>[30x]MSMYTTAQLLAANEQKFKFDPLFLRLFFRESYPFTTEKVYLSQIPGLVNMALYVSPIVSGEVIRSRGGSTSEFTPGYVKPKHEVNPQMTLRRLPDEDPQNLADPAYRRRRIIMQNMRDEELAIAQVEEMQAVSAVLKGKYTMTGEAFDPVEVDMGRSEENNITQSGGTEWSKRDKSTYDPTDDIEAYALNASGVVNIIVFDPKGWALFRSFKAVKEKLDTRRGSNSELETAVKDLGKAVSYKGMYGDVAIVVYSGQYVENGVKKNFLPDNTMVLGNTQARGLRTYGCIQDADAQREGINASARYPKNWVTTGDPAREFTMIQSAPLMLLADPDEFVSVQLA;>MKTPTIPTLLGPDGMTSLREYAGYHGGGSGFGGQLRSWNPPSESVDAALLPNFTRGNARADDLVRNNGYAANAIQLHQDHIVGSFFRLSHRPSWRYLGIGEEEARAFSREVEAAWKEFAEDDCCCIDVERKRTFTMMIREGVAMHAFNGELFVQATWDTSSSRLFRTQFRMVSPKRISNPNNTGDSRNCRAGVQINDSGAALGYYVSEDGYPGWMPQKWTWIPRELPGGRASFIHVFEPVEDGQTRGANVFYSVMEQMKMLDTLQNTQLQSAIVKAMYAATIESELDTQSAMDFILGANSQEQRERLTGWIGEIAAYYAAAPVRLGGAKVPHLMPGDSLNLQTAQDTDNGYSVFEQSLLRYIAAGLGVSYEQLSRNYAQMSYSTARASANESWAYFMGRRKFVASRQASQMFLCWLEEAIVRRVVTLPSKARFSFQEARSAWGNCDWIGSGRMAIDGLKEVQEAVMLIEAGLSTYEKECAKRGDDYQEIFAQQVRETMERRAAGLKPPAWAAAAFESGLRQSTEEEKSDSRAA[12x]

The temperate phage lambda, which infects the bacterium Escherichia coli, belongs to Siphoviridae. The virion of the lambda phage comprises an icosahedral head and a long flexible tail. The tail, which comprises the tail tube and tail tip, connects with the head through the neck. The neck–tail complex comprises a channel formed by stacked 12-fold and hexameric rings and a 3-fold symmetrical tip.

The portal occupies one of the 12 vertices of the icosahedral head. It is formed by 12 copies of gpB, which exhibits the canonical portal fold of phages belonging to the order Caudovirales. The dodecameric portal is located at a unique icosahedral vertex and facilitates the transport of DNA in and out of the head during genome packaging and delivery. The structure of gpB comprised 4 domains: wing (residues 24–249 and 368–452), stem (residues 250–279, 343–367), clip (residues 280–342), and crown (residues 453–511). The tunnel loop, which was previously indicated to facilitate the dsDNA translocation in the portal during packaging and stabilize dsDNA to avoid leakage during the phage maturation, was well resolved. The asymmetric reconstruction of the portal and capsid at a resolution of 4.0 Å showed the asymmetric interactions between the gpB and gpE subunits, as observed in the structures of phages sf6 and T4. The portal–capsid interface was analyzed using the PISA server, which revealed the salt bridges between the gpB and gpE subunits. Superimposition of the models of the 12 portal subunits revealed that a loop (residues 208–218) in the gpB wing domain underwent structural morphing to adapt to the portal–coat interactions.> GGACAUAUAAACGCGUGGAUAUGGCACGCGAGUUUCUACCGGGCACCGUAAAU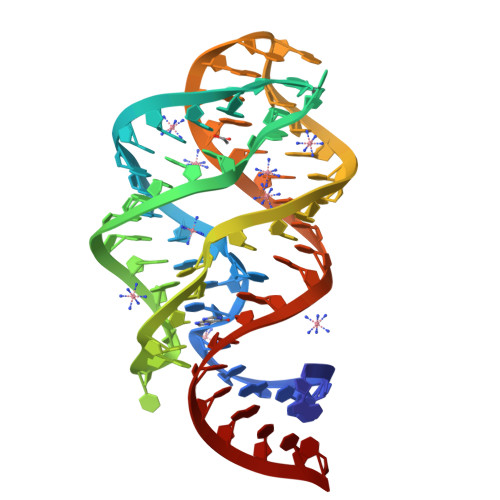GUCCGACUAUGUCC> ELTPDQQTLLHFIMDSYNKQRMPQEITNKILKEAFSAEENFLILTEMATNHVQVLVEFTKKLPGFQTLDHEDQIALLKGSAVEAMFLRSAEIFNKKLPSGHSDLLEARIRNSGISDEYITPMFSFYKSIGELKMTQEEYALLTAIVILSPDRQYIKDREAVEKLQEPLLDVLQKLCK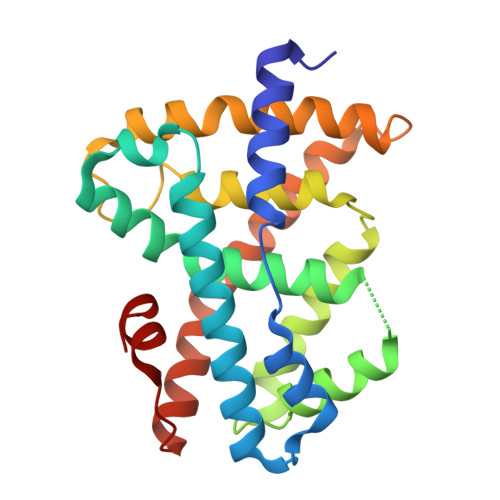IHQPENPQHFAKLLGRLTELRTFNHHHAEMLMSWRVNDHKFTPLLQEIWDV>[2x]AMKKDSKAPCVEVFDERDGCKAAGTQKASGDDGFCVKVSMKAIGFNAAEAASVTKNYGIKRFGAKSV;>[2x]MLDAFSKVITSADGKAAYVGGADLQALKKFVSEGNKRMDSVNAIVSNASCIVSDSVSGMVCENPSLIAPNGGVYTNRKMAACLRDAEIILRYVSYSLLSGDSSVLEDRCLNGLKETYASLGVPAAGNARTISIMKATVIGFITNNSQQKKLSTPAGDCSALASEVGGYFDKVSSALA;>[2x]AMKKDSKAPCVEVFDERDGCKAAGTQKASGDDGFCVKVSMKAIKMNAAEATSVTKNYNTKLL

Cryptophyte algae have a unique phycobiliprotein light-harvesting antenna that fills a spectral gap in chlorophyll absorption from photosystems. We show that the cryptophyte Hemiselmis andersenii expresses an energetically complex antenna comprising three distinct spectrotypes of phycobiliprotein, each composed of two αβ protomers but with different quaternary structures arising from a diverse α subunit family. We report crystal structures of the major phycobiliprotein from each spectrotype. We propose that the macromolecular organization of the cryptophyte antenna consists of bulk open and open-braced forms that transfer excitations to photosystems via this bridging closed form phycobiliprotein.

Four new structures of HaPE555 were determined (resolutions: 1.57 Å, 1.67 Å, 1.73 Å and 1.95 Å). The largest peak of HaPE555 (555 A) is by far the most abundant PBP constituting approximately 63% of the overall protein complement (with other HaPE555 spectrotype peaks contributing 8%). All five crystal forms of protein HaPE555 are constructed from continuous filaments of PBPs, which are organized into two-dimensional rafts. The filaments are generated via knobs-into-holes packing but differ in the distances between adjacent molecules along the filament (having either tight or loose interfaces). This packing brings the chromophores of neighboring PBPs closer together increasing the possibility of energy transfer. The bulk antenna proteins, HaPE555 and HaPE560, are densely packed to form a concentrated glass of proteins as evidenced by electron micrographs and FRAP experiments. It is also possible that the rafts of HaPE555 filaments seen in all crystal forms are part of the organizing principle of the antenna architecture. We have shown that HaPE555 and HaPE560 form the bulk of the light harvesting antenna (roughly 6/7 of the PBPs) and capture the highest energy photons. Thus, HaPE555 and HaPE560 have evolved to capture photons that would be otherwise lost by the integral membrane photosystems: they plug a spectral hole.>GSGAMRIGMVCPYSFDVPGGVQSHVLQLAEVLRDAGHEVSVLAPASPHVKLPDYVVSGGKAVPIPYNGSVARLRFGPATHRKVKKWIAEGDFDVLHIHEPNAPSLSMLALQAAEGPIVATFHTSTTKSLTLSVFQGILRPYHEKIIGRIAVSDLARRWQMEALGSDAVEIPNGVDVASFADAPLLDGYPREGRTVLFLGRYDEPRKGMAVLLAALPKLVARFPDVEILIVGRGDEDELREQAGDLAGHLRFLGQVDDATKASAMRSADVYCAP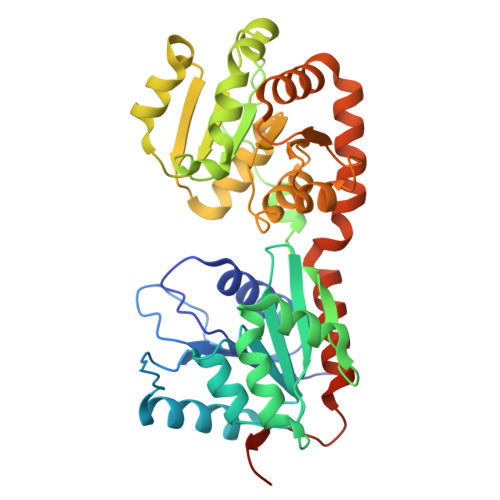HLGGESFGIVLVEAMAAGTAVVASDLDAFRRVLADGDAGRLVPVDDADGMAAALIGILEDDQLRAGYVARASERVHRYDWSVVSAQIMRVYETVSGAGIKVQVSGAANRDETAGESV[4x]(1S,3R,5Z,7E,14beta,17alpha,23R)-23-(2-hydroxy-2-methylpropyl)-20,24-epoxy-9,10-secochola-5,7,10-triene-1,3-diol 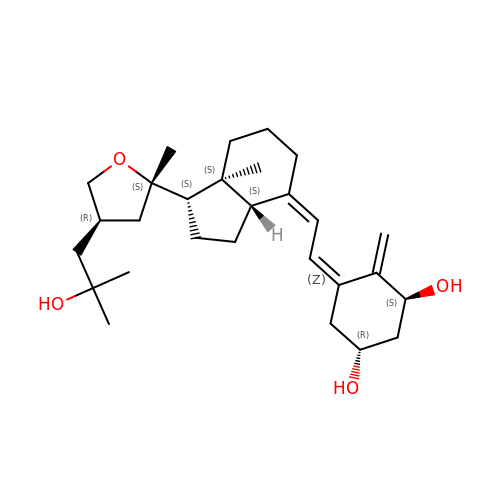| C28 H44 O4 | QFEREDUWILIRPI-FOPXFMLJSA-N> M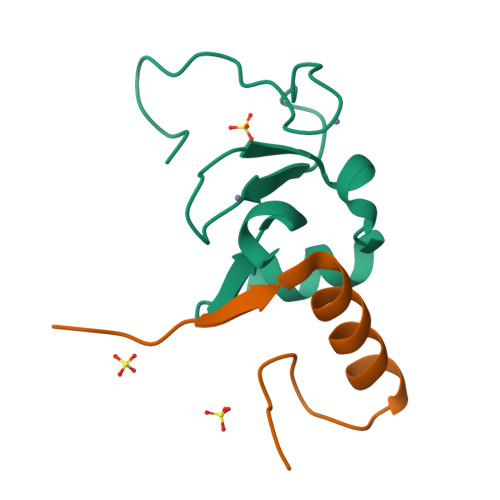GHSSSDPVYPCGICTNEVNDDQDAILCEASCQKFFHRICTGMTETAYGLLTAEASAVWGCDTCMADKDVQ;> AAKVVYVFSTEMANKAAEAVLKGQVETIVSFHI> SNASADAQSFLNRVCGVSAARLTPCGTGTSTDVVYRAFDIYNDKVAGFAKFLKTNCCRFQEKDEDDNLIDSYFVVKRHTFSNYQHEETIYNLLKDCPAVAKHDFFKFRIDGDMVPHISRQRLTKYTMADLVYALRHFDEGNCDTLKEILVTYNCCDDDYFNKKDWYDFVENPDILRVYANLGERVRQALLKTVQFCDAMRNAGIVGVLTLDNQDLNGNWYDFGDFIQTTPGSGVPVVDSYYSLLMPILTLTRALTAESHVDTDLTKPYIKWDLLKYDFTEERLKLFDRYFKYWDQTYHPNCVNCLDDRCILHCANFNVLFSTVFPPTSFGPLVRKIFVDGVPFVVSTGYHFRELGVVHNQDVNLHSSRLSFKELLVYAADPAMHAASGNLLLDKRTTCFSVAALTNNVAFQTVKPGNFNKDFYDFAVSKGFFKEGSSVELKHFFFAQDGNAAISDYDYYRYNLPTMCDIRQLLFVVEVVDKYFDCYDGGCINANQVIVNNLDKSAGFPFNKWGKARLYYDSMSYEDQDALFAYTKRNVIPTITQMNLKYAISAKNRARTVAGVSICSTMTNRQFHQKLLKSIAATRGATVVIGTSKFYGGWHNMLKTVYSDVENPHLMGWDYPKCDRAMPNMLRIMASLVLARKHTTCCSLSHRFYRLANECAQVLSEMVMCGGSLYVKPGGTSSGDATTAYANSVFNICQAVTANVNALLSTDGNKIADKYVRNLQHRLYECLYRNRDVDTDFVNEFYAYLRKHFSMMILSDDAVVCFNSTYASQGLVASIKNFKSVLYYQNNVFMSEAKCWTETDLTKGPHEFCSQHTMLVKQGDDYVYLPYPDPSRILGAGCFVDDIVKTDGTLMIERFVSLAIDAYPLTKHPNQEYADVFHLYLQYIRKLHDELTGHMLDMYSVMLTNDNTSRYWEPEFYEAMYTPHTVLQ;>[2x]SNAAIASEFSSLPSYAAFATAQEAYEQAVANGDSEVVLKKLKKSLNVAKSE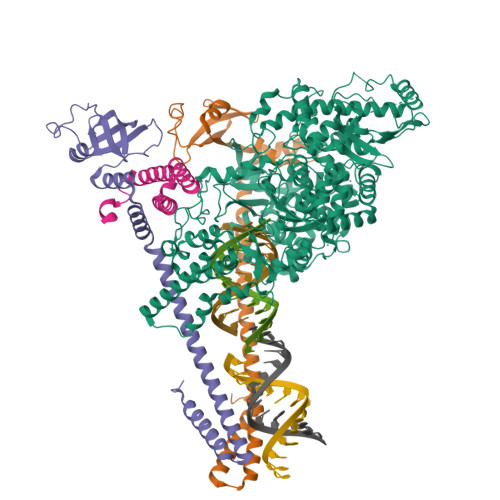FDRDAAMQRKLEKMADQAMTQMYKQARSEDKRAKVTSAMQTMLFTMLRKLDNDALNNIINNARDGCVPLNIIPLTTAAKLMVVIPDYNTYKNTCDGTTFTYASALWEIQQVVDADSKIVQLSEISMDNSPNLAWPLIVTALRANSAVKLQ;> SNASKMSDVKCTSVVLLSVLQQLRVESSSKLWAQCVQLHNDILLAKDTTEAFEKMVSLLSVLLSMQGAVDINKLCEEMLDNRATLQ> MLV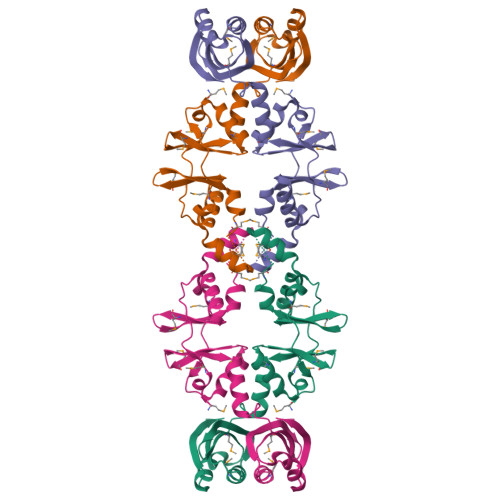RDWMTKDPVVVAPDTPVLEAIRLLKEKGFRRLPVMEGGRLVGLVTDKDLKDAMPSKATTLSVWEMNYLLAKLTVREVMARPVVTVEADAPLEKAALLMEERKIGGLPVMEGERLVGIITVTDVLRAFIEVLGLKLGGLRITVDIPDVPGALAQMAQAVPPANIVSIATAAHLPGYQRLVMRVVGEDVEGVPKRLEAAGERVVDVRPG>[2x]XEVEALEKKVEALEAKV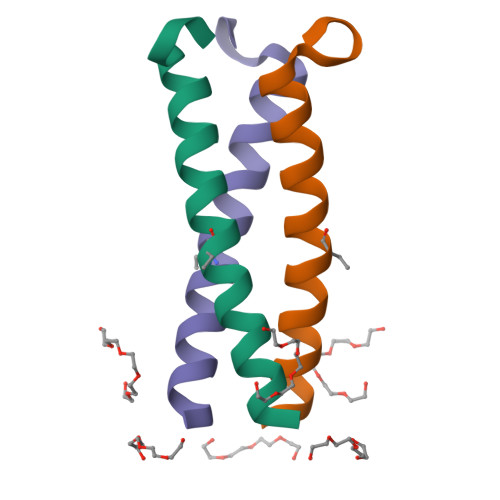QKLEKKVEALEHGWDGR> PISPIETVPVKLKPGMDGPKVKQWPLT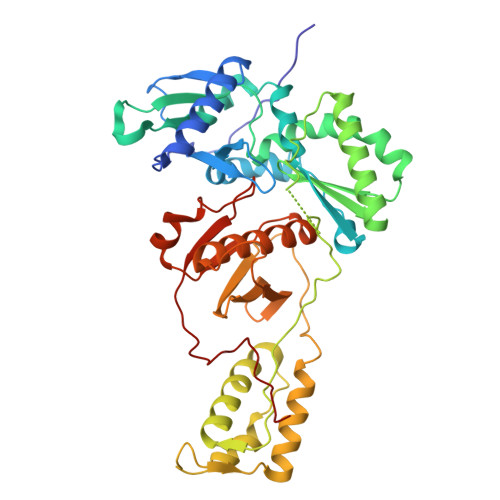EEKIKALVEICTEMEKEGKISKIGPENPYNTPVFAIKKKDSTKWRKLVDFRELNKRTQDFWEVQLGIPHPAGLKKKKSVTVLDVGDAYFSVPLDEDFRKYTAFTIPSINNETPGIRYQYNVLPQGWKGSPAIFQSSMTKILEPFKKQNPDIVIYQYMDDLYVGSDLEIGQHRTKIEELRQHLLRWGLTTPDKKHQKEPPFLWMGYELHPDKWTVQPIVLPEKDSWTVNDIQKLVGKLNWASQIYPGIKVRQLSKLLRGTKALTEVIPLTEEAELELAENREILKEPVHGVYYDPSKDLIAEIQKQGQGQWTYQIYQEPFKNLKTGKYARMRGAHTNDVKQLTEAVQKITTESIVIWGKTPKFKLPIQKETWETWWTEYWQATWIPEWEFVNTPPLVKLWYQGGHHHHHHH> IQINQVRPKLPLLKILHAAGAQG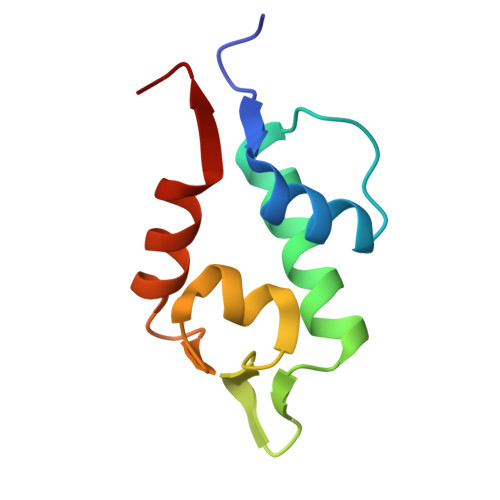EMFTVKEVMHYLGQYIMVKQLYDQQEQHMVYCGGDLLGELLGRQSFSVKDPSPLYDMLRKNLVTLAT>TVPASVDWRKKGAVTSVKDQGQCGSCWAFSTIVAVEGINQIKTNKLVSLSEQELVDCDTDQNQGCNGGLMDYAFEFIKQRGGITTEANYPYEAYDGTCDVSKENAPAVSIDGHENVPENDENALLKAVANQPVSVAIDAGGSDFQFYSEGVFTGSCGTELDHGVAIVGYGTTIDGTKYWTVKNSWGPEWGEKGYIRMERGISDKEGLCGIAMEAS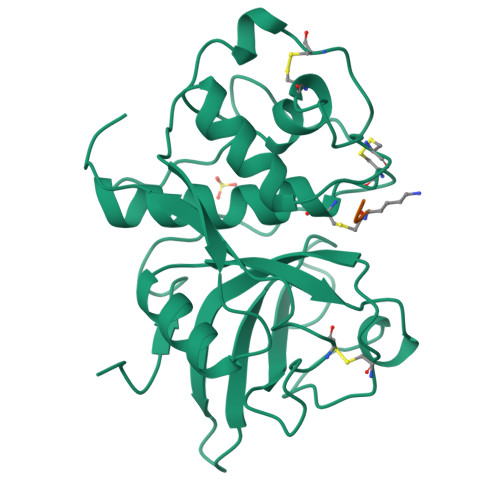YPIKKSSNNPSGIK[2x]> GSGDSGSPGGTYINN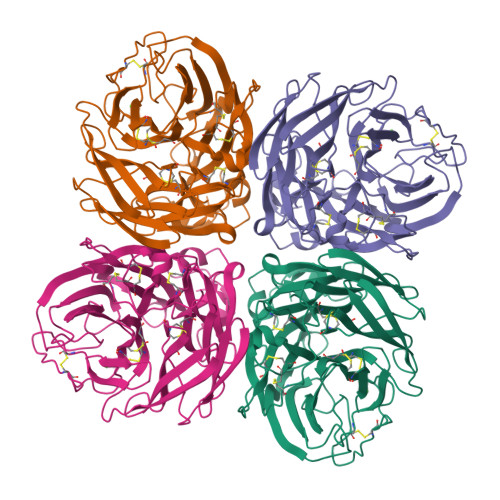TEPICDVKGFAPFSKDNGIRVGSRGHIFVIREPFVSCSPVGCRTFFLTQGSLLNDKHSNGTVKDRSPFRTLMSVEVGQSPNVYQARFEAVAWSATACHDGKKWMAIGVTGPDSKAVAVVHYGGVPTDVVNSWAGDILRTQESSCTCIQGNCYWVMTDGPANRQAQYRIYKANQGKIIGRKDVSFSGGHIEECSCYPNDGKVECVCRDNWTGTNRPVLIISPDLSYRVGYLCAGLPSDTPRGEDTQFVGSCTSPMGNQGYGVKGFGFRQGTDVWVGRTISRTSRSGFEIIRIKNGWTQTSKEQIRRQVVVDNSNWSGYSGSFTLPVELSGRECLVPCFWVEMIRGRPEERTIWTSSSSIVMCGVDYEIADWSWHDGAILPFDIDKM> MNYNLSKYPDDVSRLFKPRPPLSYKRPTDYPYAKRQTNPNITGVANLLSTSLKHYMEEFPEGSPNNHLQRYEDIKLSKIKNAQLLDRRLQNWNPNVDPHIKDTDPYRTIFIGRLPYDLDEIELQKYFVKFGEIEKIRIVKDKITQKSKGYAFIVFKDPISSKMAFKEIGVHRGIQIKDRICIVDIERGRTVKYFKPRRLGGGLGGRGYSNRDSRLPGRFASASTSNPAERNYAPRLPRRETSSSAYSADRYGSSTLDARYRGNRPLLSAATP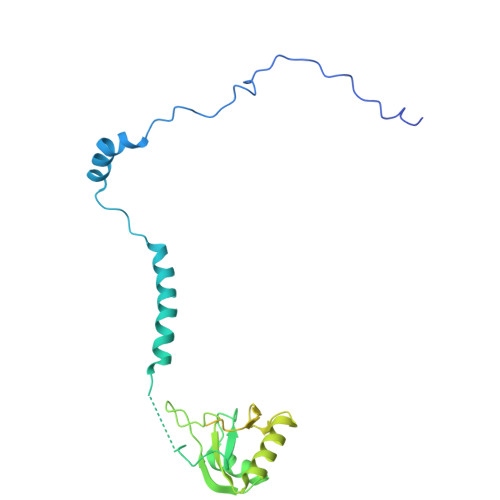TAAVTSVYKSRNSRTRESQPAPKEAPDY>MHVNGKVALVTGAAQGIGRAFAEALLLKGAKVALVDWNLEAGVQCKAALDEQFEPQ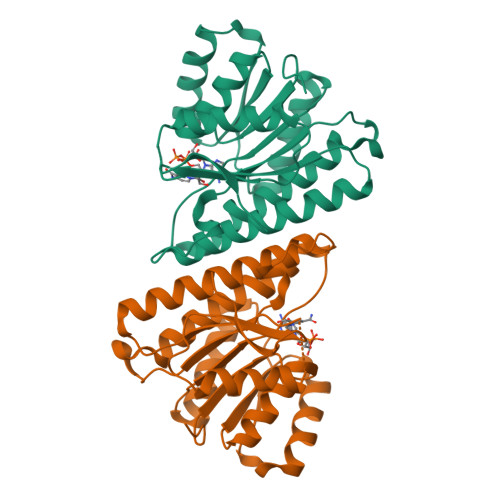KTLFIQCDVADQQQLRDTFRKVVDHFGRLDILVNNAGVNNEKNWEKTLQINLVSVISGTYLGLDYMSKQNGGEGGIIINMSSLAGLMPVAQQPVYCASKHGIVGFTRSAALAANLMNSGVRLNAICPGFVNTAILESIEKEENMGQYIEYKDHIKDMIKYYGILDPPLIANGLITLIEDDALNGAIMKITTSKGIHFQDY[2x]Unlike other chromatin remodelers, INO80 preferentially mobilizes hexasomes, which can form during transcription. Here, we report cryogenic-electron microscopy (cryo-EM) structures of endogenously purified S. cerevisiae INO80 bound to a hexasome and a nucleosome. We group subunits of the INO80 complex into four modules: Rvb module (Rvb1/Rvb2), Arp8 module (Arp8/Arp4/Actin/Ies4 and Taf14), Ino80 module (Ino80/Ies2) and Arp5 module (Arp5/Ies6). The Ino80 protein consists of three major regions: the N-terminal domain (NTD), the HSA region (Ino80HSA) and the ATPase domain (Ino80ATPase).

In contrast, the states of INO80 bound to a nucleosome have Ino80ATPase bound near either SHL-6 or −7 consistent with previous findings. In contrast, consistent with prior findings, we observe that Ino80ATPase engages the nucleosome near two positions, SHL-7 and −6. All Ino80ATPase locations on hexasomes are different than on nucleosomes, which are near SHL-6 or SHL-7 (12-14). Also as previously proposed, our findings are consistent with the possibility that Ino80ATPase acts near SHL-6 when sliding nucleosomes. Here we show that site-specific gaps near SHL-2 or SHL-6 substantially inhibit INO80’s sliding of nucleosomes (by ~200 fold). The pause could represent the reorientation of Ino80ATPase from SHL-6/−7 towards SHL-2 and add a step that slows remodeling of nucleosomes compared to hexasomes. For such a scenario we speculate that Ino80ATPase translocates DNA near SHL-6 and effective translocation also requires action of the Arp5 module near SHL-2 as previously proposed.

> IEIDVLCDLTQRQAKLYQVLKSQISTNYDAIENAATNDSTSNSASNSGSDQNLINAVMQFRKVCNHPDLFERADVDSPFSFTTFGKTTSMLTASVANNNSSVISNSNMNLSSMSSNNISNGKFTDLIYSSRNPIKYSLPRLIYEDLILPNYNNDVDIANKLKNVKFNIFNPSTNYELCLFLSKLTGEPSLNEFFRVSTTPLLKRVIERTNGPKNTDSLSFKTITQELLEVTRNAPSEGVMASLLNVEKHAYEREYLNCIQRGYHPNVSAPPVTIEVLGSSHVTNSINNELFDPLISQALSDIPAITQYNMHVKKGIPVEDFPKTGLFPEPLNKNFSSNISMPSMDRFITESAKLRKLDELLVKLKSEGHRVLIYFQMTKMMDLMEEYLTYRQYNHIRLDGSSKLEDRRDLVHDWQTNPEIFVFLLSTRAGGLGINLTAADTVIFYDSDWNPTIDSQAMDRAHRLGQTRQVTVYRLLVRGTIEERMRDRAKQKE;> MSSRDASLTPLKAVVIDDPPLRQTPEPFDEQSAYNPQSPIAIDFGSSKLRAGFVNHATPTHIFPNALTKFRDRKLNKNFTFVGNDTLLDQAVRSQSRSPFDGPFVTNWNLTEEILDYTFHHLGVVPDNGIPNPILLTERLATVQSQRTNWYQILFETYNVPGVTFGIDSLFSFYNYNPSGNKTGLVISCGHEDTNVIPVVDGAGILTDAKRINWGGHQAVDYLNDLMALKYPYFPTKMSYLQYETMYKDYCYVSRNYDEDIEKILTLENLDTNDVVVEAPFTEVLQPQKTEEELRIQAEKRKETGKRLQEQARLKRMEKLVQKQEEFEYFSKVRDQLIDEPKKKVLSVLQNAGFDDERDFKKYLHSLEQSLKKAQMVEAEDDSHLDEMNEDKTAQKFDLLDIADEDLNEDQIKEKRKQRFLKASQDARQKAKEEKERVAKEEEEKKLKEQQWRETDLNGWIKDKRLKLNKLIKRRKEKLKLRDEMKDRKSQVSQNRMKNLASLAEDNVKQGAKRNRHQATIDNDPNDTFGANDEDWLIYTDITQNPEAFEEALEYEYKDIVELERLLLEHDPNFTEEDTLEAQYDWRNSILHLFLRGPRPHDSENIHEQHQMHLNVERIRVPEVIFQPTMGGQDQAGICELSETILLKKFGSQPGKLSQTSIDMVNNVLITGGNAKVPGLKERIVKEFTGFLPTGTNITVNMSSDPSLDAWKGMAALARNEEQYRKTVISKKEYEEYGPEYIKEHKLGNTKYFED;> ERLLFLRSVGERNEIGFPSRFKSAHYKKPTRRHKSARQLISDENKRINALLTKANKAAESSTAARRLVPKATYFSVEAPPSIRPAKKYCDVTGLKGFYKSPTNNIRYHNAEIYQLIVKPMAPGVDQEYLKLRGAN;>[3x]VTRTAAHTHIKGLGLDESGVAKRVEGGFVGQIEAREACGVIVDLIKAKKMSGRAILLAGGPSTGKTALALAISQELGPKVPFCPLVGSELYSVEVKKTETLMENFRRAIGLRIKETKEVYEGEVTELTPEDAENPLGGYGKTISHVIVGLKSAKGTKTLRLDPTIYESIQREKVSIGDVIYIEANTGAVKRVGRSDAYATEFDLETEEYVPLPKGEVHKKKEIVQDVTLHDLDVANARPQGGQDVISMMGQLLKPKKTEITEKLRQEVNKVVAKYIDQGVAELIPGVLFIDEVNMLDIEIFTYLNKALESNIAPVVVLASNRGMTTVRGTEDVISPHGVPPDLIDRLLIVRTLPYDKDEIRTIIERRATVERLQVESSALDLLATMGTETSLRYALQLLAPCGILAQTSNRKEIVVNDVNEAKLLFLDAKRSTKILETSANYL;>[3x]KSLSLIAAHSHITGLGLDENLQPRPTSEGMVGQLQARRAAGVILKMVQNGTIAGRAVLVAGPPSTGKTALAMGVSQSLGKDVPFTAIAGSEIFSLELSKTEALTQAFRKSIGIKIKEETELIEGEVVEIQIDRSITGGHKQGKLTIKTTDMETIYELGNKMIDGLTKEKVLAGDVISIDKASGKITKLGRSFARSRDYDAMGADTRFVQCPEGELQKRKTVVHTVSLHEIDVINSRTQGFLALFTGDTGEIRSEVRDQINTKVAEWKEEGKAEIVPGVLFIDEVHMLDIECFSFINRALEDEFAPIVMMATNRGVSKTRGTNYKSPHGLPLDLLDRSIIITTKSYNEQEIKTILSIRAQEEEVELSSDALDLLTKTGVETSLRYSSNLISVAQQIAMKRKNNTVEVEDVKRAYLLFLDSARSVKYVQENESQYIDDQGNVQISIAK;> FVKPRRPYNSEGMTRILRRYEEDLFCTF> GSSHHHHHHSSGENLYFQSGSHYKQLIKNDENITVNESVPRGRILDRNGKVLVDNASKMSITYTRNRKTSQKEMLNTAKKLTDLIKMDTDKITERDKKDFWIQMYPSSAKKLMRKEQLMLEDGSISQDQFDTQLRDKIGKKQLKQLTKKDLQVLAIYREMNAGSTLDPQTIKNEDVSEKEYAAVSQQLSKLPGVNTTMDWDRKYPYGDTLRGIFGDVSTSTEGIPKELTEQYLSKGYSRNDRVGKSYLEYQYEDVLKGTKKQMKYTTDKSGRVISSEVLNPGSRGHDLQLTIDIDLQKKVESLLEKQISKLRSQGAKDMDNALMVVQNPKNGDILAIAGKQIDKQGKLKDYDIGNFTAQYTVGSSVKGGTLLAGYQNKAINVGETMVDEPLKFQGGLTKRSYFNKNGHVSIDDKQALMHSSNVYMFKTALKLAGDPYTSGMSLPNNIADAGRKLRKGLNQVGLGLKTGIDLPNETPGQIEPLTNNPGNYLDLAIGQYDTYTPLQLSQYVSTIANDGYRIQPHIGLSIYESTNKDETGPLKRKIKGNVLNKVNNSNDEIKEVQEGFKMAFNEKQGTGYASFRNTVVPSAGKTGTAEVFQDGEPRVNSTYIGYAPVDDPKLSFSIVYTNQPVPPPWLN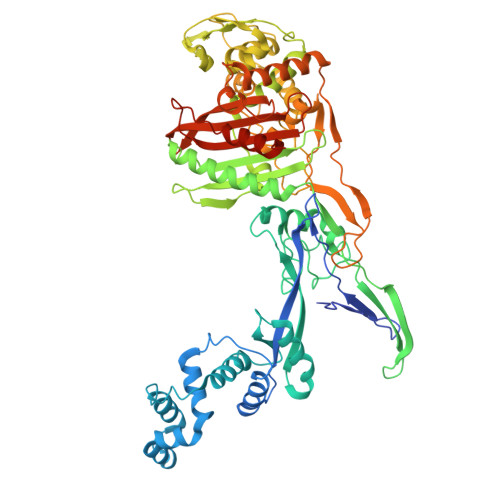GGDLGRDVINYYFKDKDNKKDDSQSNNEEKED>MAIPEEFDILVLGGGSSGSCIAGRLANLDHSLKVGLIEAGENNLNNPWVYLPGIYPRNMKLDSKTASFYTSNPSPHLNGRRAIVPCANVLGGGSSINFMMYTRGSASDYDDFQAEGWKTKDLLPLMKKTETYQRACNNPDIHGFEGPIKVSFGNYTYPVCQDFLRASESQGIPYVDDLEDLVTAHGAEHWLKWINRDTGRRSDSAHAFVHSTMRNHDNLYLICNTKVDKIIVEDGRAAAVRTVPSKPLNPKKPSHKIYRARKQIVLSCGTISSPLVLQRSGFGDPIKLRAAGVKPLVNLPGVGRNFQDHYCFFSPYRIKPQYESFDDFVRGDAEIQKRVFDQWYANGTGPLATNGIEAGVKIRPTPEELSQMDESFQEGYREYFEDKPDKPVMHYSIIAGFFGDHTKIPPGKYMTMFHFLEYPFSRGSIHITSPDPYAAPDFDPGFMNDERDMAPMVWAYKKSRETARRMDHFAGEVTSHHPLFPYSSEARALEMDLETSNAYGGPLNLSAGLAHGSWTQPLKKPTAKNEGHVTSNQVELHPDIEYDEEDDKAIENYIREHTETTWHCLGTCSIGPREGSKIVKWGGVLDHRSNVYGVKGLKVGDLSVCPDNVGCNTYTTALLIGEKTATLVGEDLGYSGEALDMTVPQFKLGTYEKTGLARF[8x]

The methanol assimilation pathway is initiated by the oxidation of that alcohol to formaldehyde. This reaction is catalyzed by the FAD-dependent alcohol oxidase (AOX; EC 1.1.3.13), which belongs to the family of glucose-methanol-choline (GMC) oxidoreductases. Like other members of the glucose-methanol-choline (GMC) oxidoreductase superfamily, AOX1 exhibits the characteristic two-domains topology of the PHBH fold, containing a FAD-binding domain (residues 1–155, 192–306 and 568–663) and a substrate-binding domain (residues 156–191 and 307–567). The mature active form of AOX1 is an oligomer comprising eight identical subunits, each carrying one non-covalently bound flavin adenine dinucleotide (FAD) molecule as prosthetic group.

The final model of AOX1 was refined at a resolution of 2.35 Å to R and Rfree factors of 0.1774 and 0.2049, respectively. Analysis of the crystal packing revealed that P. pastoris AOX1 crystallized as a homo-octamer with approximate dimensions of 121.8 Å x 133.8 Å x 134.5 Å, which is consistent with previous studies on the AOX oligomerization based on ultracentrifugation and electron microscopy. The octamer appears to be a tetramer of dimers, but can also be described as two tetramers positioned face to face to each other. The two tetramers interact exclusively via the substrate binding domains, while the FAD binding domains occupy the outer surface of the oligomer. Comparison with the structure of CO, the most closely related structural homolog, indicates that formation of the observed oligomerization state of AOX1 is mainly facilitated by insertions involved in numerous interactions between monomers (residues 326–351, 486–548, 247–251, 638–663). Interestingly upon enzyme oligomerization the PTS (residues 660–663) gets buried inside the octamer. Interestingly, the omit mFo-DFc difference electron density map contoured at 3.5 sigma level clearly indicates presence of a modified FAD, in which the configuration of the C2’ carbon of the sugar chain attached to the isoalloxazine ring is changed from R to S, hence being an arabityl rather than a ribityl chain. Importantly, the change in chiral configuration at atom C2’ in AOX’s FAD results in the formation of a new intramolecular hydrogen bond between the arabityl C2’ OH group of the modified a-FAD and the N1 atom of the isoalloxazine ring system, which most likely modulates the redox potential of the FAD cofactor. Analysis of the crystal structure of AOX1 reveals that the active site is completely solvent inaccessible. Importantly, the substrate-binding pocket of AOX1 is reduced in size with regard to CO, due to the replacement of CO Ser101 to AOX1 Phe98, CO Tyr465 to AOX1 Trp 566, and CO Thr 376 to AOX1 Phe417, and in addition is more hydrophobic what could explain the preference for methanol as substrate.> SKGLQIRVQGLDEAQEFYELESKADGQLLLSDVFRRINLIESDYFGLEFQNLQMNWVWLDPSKLIVKQVRRPMNTLFRLSVKFFPPDPGQLQEEFTRYLFSLQIKRDLLDGRLSCTENTAALLASHLVQSEIGDYDDLADREFLKMNKLLPCQEHVQEKIMELHRRHTGQTPAESDFQVLEIARKLEMFGVRFHPAADREGTKINLAVAHMGLQVFQGHTKINTFNWSKIRKLSFKRKRFLIKLHPEVHGPHQDTLEFLMGSRDQCKIFW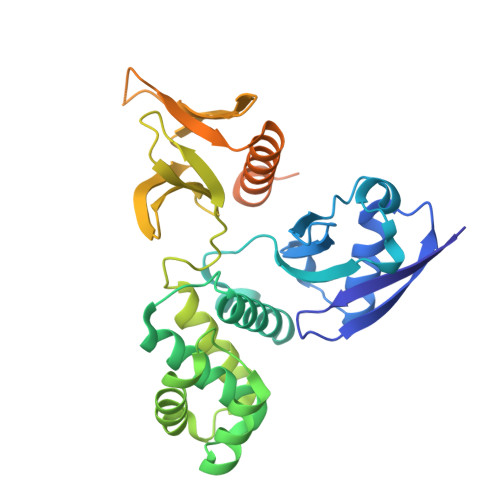KNCVEHHSFFRLLDQPQPKSKAIFFSRGSSFRYSGRTQKQLVEYVRDSGLRRTPYQRRNSKIR>[4x]GSMNTPNGNSLSAAELTCGMIM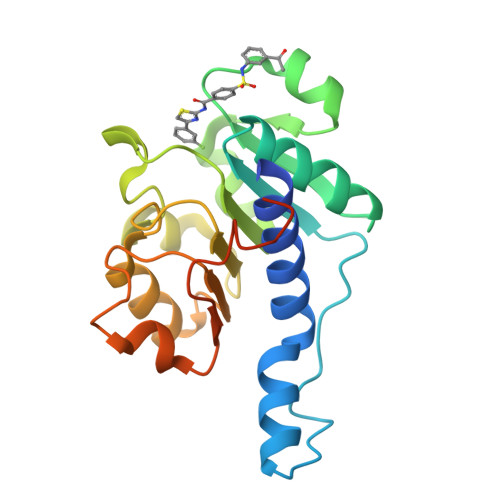CLARQIPQATASMKDGKWERKKFMGTELNGKTLGILGLGRIGREVATRMQSFGMKTIGYDPIISPEVSASFGVQQLPLEEIWPLCDFITVHTPLLPSTTGLLNDNTFAQCKKGVRVVNCARGGIVDEGALLRALQSGQCAGAALDVFTEEPPRDRALVDHENVISCPHLGASTKEAQSRCGEEIAVQFVDMV>[8x]QPVTGGAEALRIRWSKAPCRFCGTGCGVMVGTRDGQVVATHGDTQAEVNRGLNCVKGYFLSKIMYGEDRLTTPLLRMKDGVYHKEGEFAPVSWDEAFDVMAAQAK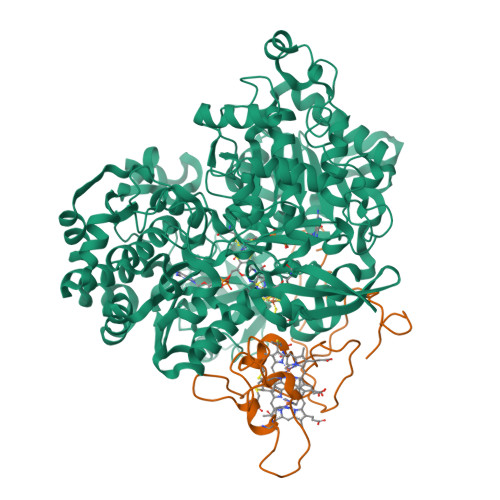LVLKEKAPEAVGMFGSGQWTIWEGYAASKLMRAGFRSNNLDPNARHCMASAATAFMRTFGMDEPMGCYDDFEAADAFVLWGSNMAEMHPILWSRLTDRRLSHEHVRVAVLSTFTHRSSDLSDTPIIFRPGTDRAILNYIAHHIISTGRVNRDFVDRHTNFALGATDIGYGLRPEHQLQLAAKGAADAGAMTPTDFETFAALVSEYTLEKAAEISGVEPALLEELAELYADPDRKWMSLWTMGFNQHVRGVWANHMVYNLHLLTGKISEPGNSPFSLTGQPFACGTAREVGTFAHRLPADMVVTNPEHRAHAEEIWKLPAGLLPDWVGAHAVEQDRKLHDGEINFYWVQVNNNMQAAPNIDQETYPGYRNPENFIVVSDAYPTVTGRAADLVLPAAMWVEKEGAYGNAERRTHFWHQLVEAPGEARSDLWQLMEFSKRFTTDEVWPEEILSAAPAYRGKTLFEVLFANGSVDRFPASDVNPDHANHEAALFGFYPQKGLFEEYAAFGRGHGHDLAPFDTYHEVRGLHWPVVEGEETRWRYREGFDPYVKPGEGLRFYGKPDGRAVILGVPYEPPAESPDEEFGFWLVTGRVLEHWHSGSMTLRWPELYKAFPGAVCFMHPEDARSRGLNRGSEVRVISRRGEIRTRLETRGRNRMPRGVVFVPWFDASQLINKVTLDANDPISRQTDFKKCAVKIEAV;>[8x]QDAPRLTGADRPMSEVAAPPLPETITDDRRVGRNYPEQPPVIPHSIEGYQLSVNANRCLECHRRQYSGLVAAPMISITHFQDREGQMLADVSPRRYFCTACHVPQTNAQPLVTNEFRDMLTLMPASNEAE adenosine 3',5'-bis(trihydrogen diphosphate) | C10 H17 N5 O16 P4 | 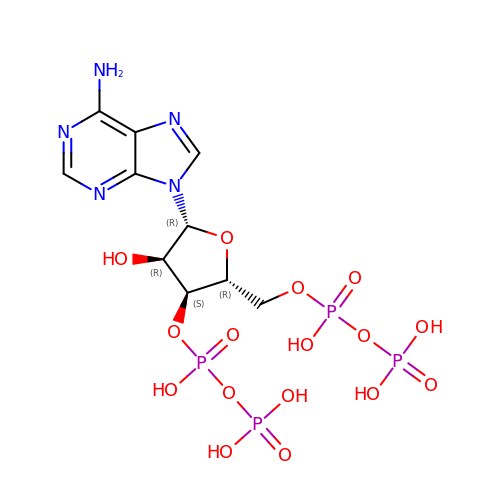DWZMGWMGGHNJLF-KQYNXXCUSA-N> AE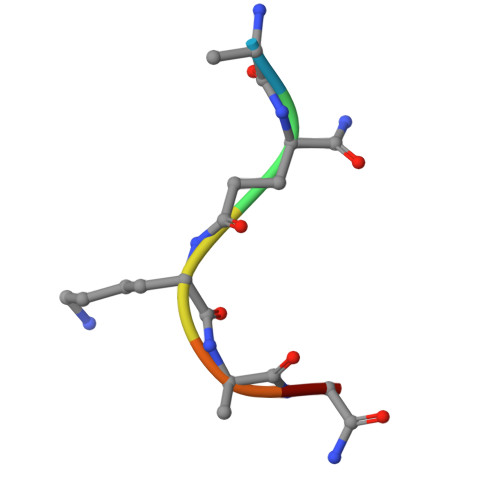KAAX>MELRVGNRYRLGRKIGSGSFGDIYLGTDIAAGEEVAIKLECVKTKHPQLHIESKIYKMMQGGVGIPTIRWCGAEGDYNVMVMELLGPSLEDLFNFCSRKFSLKTVLLLADQMISRIEYIHSKNFIHRDVKPDNFLMGLGKKGNLVYIIDFGLAKKYRDARTHQHIPYRENKNLTGTARYASINTHLGIEQSRRDDLESLGYVLMYFNLGSLPWQGLKAATKRQKYERISEKKMSTPIEVLCKGYPSEFATYLNFCRSLRFDDKPDYSYLRQLFRNLFHRQGFSYDYVFDWNMLKFGASRAA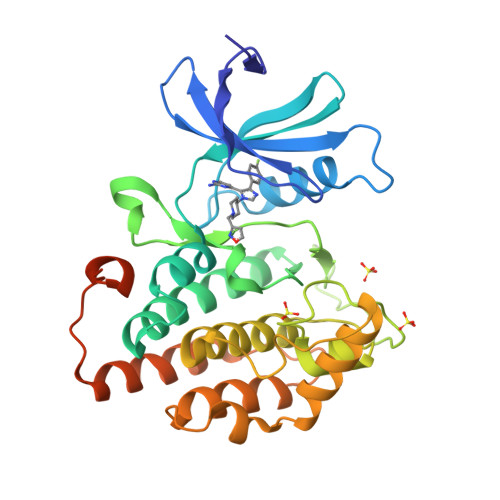LVPRGSPGGGSHHHHHH[2x]> ETGVALEQRPISITRNAKQSASLNCKILNPVSDYVHWYRSQEGRAPERLLVYSRSKSESVPDPGFSADKVRAY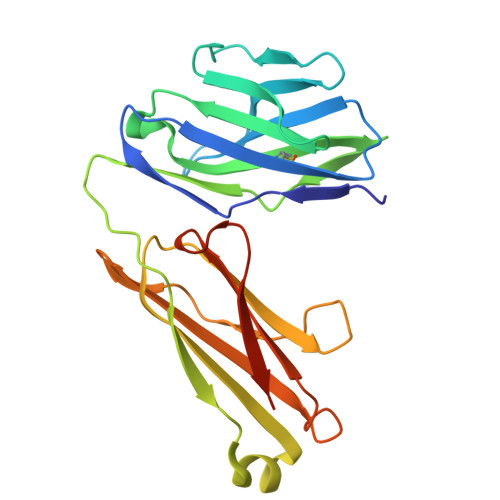KGADDTCRLIVSDLQVSDSGVYHCASWDGRVKVFGEGTRLIVTESAFKKKPPKPIFFLPTSEEIKQKQSGTYICLLEDFFPNVVKTYWKEDGNSQPLDAQFGPITGGGNSYSQVSWLTVKEDVLRKNLTYFYQHEDLGMEPKAFSISSVREKGSLVPR>EQLTKCEVFQ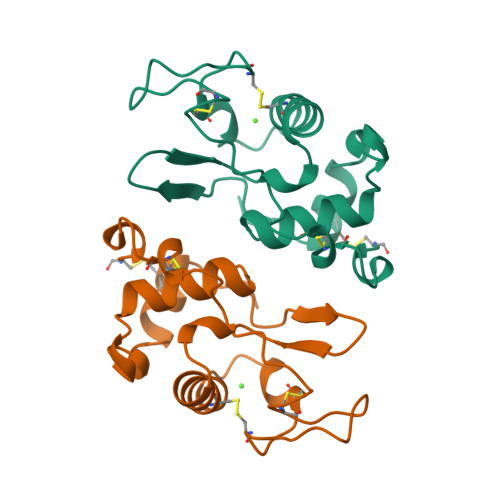KLKDLKDYGGVSLPEWVCTAFHTSGYDTQAIVQNNDSTEYGLFQINNKIWCKDDQNPHSRNICNISCDKFLDDDLTDDIVCAKKILDKVGINYWLAHKALCSEKLDQWLCEKL[2x]2-(1-methylethyl)imidazo[1,2-b]pyridazin-6-ol | C9 H11 N3 O | 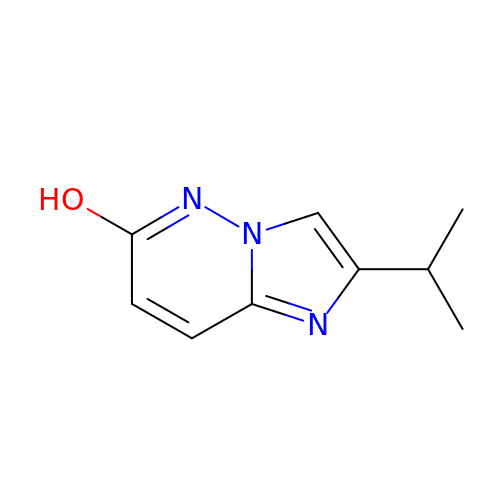QAOPIBXTQUXLFU-UHFFFAOYSA-N>[3x]MMQQSRPASDPQVVEAARKEGRLIIYSSTDQSSAQALLDDFRKLYPFIQIEYNDLGTQAIYDRFVSETAAGASSADLLWSSAMELQVKLASEGYALPYDSPEAKNWPANARLGNLAYSTTLEPAVVVYNKRFLKPEEVPTTREGLAR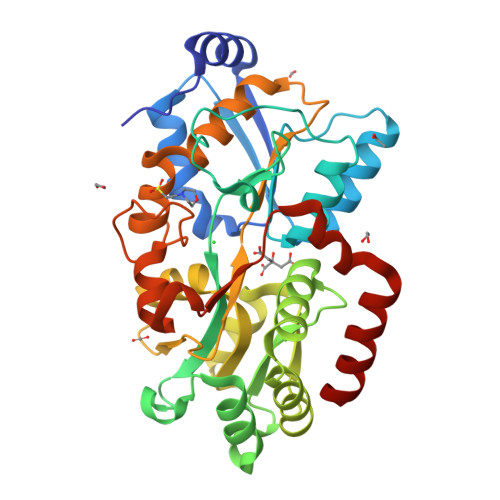LLQEPRMRGRVATWDPERSAVGFTILKADYDRFPAFQELARAFGKAQAALYSSTGAAFEKVISGEHYLAYGFFGSYALLRQRTVKDLGIAYLTDGTVAIQRVAFINKRAAHPNAAKLFLDYLLSLRGQNLMAYTALIFARRETVVGEATPQALYKAVGGKDKVYAIPVSTEILKNLDPAERMRFLTFWRQAVRGQ>CGTATACG[4x]

In this study, we used d(CGTATACG)2, which forms a tetraplex base-pair junction that resembles the DNA–DNA contact structure, as a model target for two alkyl-linked diaminoacridine bis-intercalators, DA4 and DA5. To explore the possibility of targeting inter-DNA duplex structures, we synthesized two acridine-based derivatives, DA4 and DA5, by coupling 9-aminoacridine moieties with hydrocarbon chains of four and five atoms, respectively. Cross-linking of the junction site by the bis-intercalators induced substantial structural changes in the DNA, transforming it from a B-form helical end-to-end junction to an over-wounded side-by-side inter-duplex conformation with A-DNA characteristics and curvature. Furthermore, we have shown that the different topological changes induced by DA4 and DA5 lead to the inhibition of topoisomerase 2 activities, which may account for their antitumor effects.

To understand the structural basis of the binding of DA4 and DA5, we determined the crystal structures of DA4 and DA5 with the d(CGTATACG)2 sequence in the C2221 and P21 space groups, respectively, at a resolution of 1.58 Å. In contrast, the asymmetric unit of the DA5–DNA complex contains two independent duplexes, each intercalated by a single DA5 moiety and two Mg2+ ions, which form octahedral coordination with five water molecules and one phosphate oxygen from the thymine bases. In contrast to the unliganded DNA structure, the crystal assembly of the DA4–DNA and DA5–DNA complexes revealed that the duplexes were juxtaposed near terminal CpG sites (C1pG2 and C7*pG8*, respectively), with DA4 and DA5 bis-intercalating into neighboring duplexes. The four-carbon linker of DA4 adopted a relatively straight conformation, in contrast to the five-carbon linker of DA5, which bent toward the DNA backbone. In the DA4–DNA complex, the two chromophores formed an angle of ∼60° with the horizontal plane of the acridine ring, whereas in the DA5–DNA complex, the angle between the two acridine chromophores was ∼50°. This flexibility in the DA5 linker resulted in its chromophore aligning in an optimal position to form continuous stacking interactions with DNA base pairs. A detailed analysis revealed that, compared to DA4, the bending of the DA5 linker resulted in more π–π stacking interactions with DNA bases. Furthermore, amino nitrogen at carbon 9 of acridine in DA5 showed a direct water-mediated interaction with cytosines C1 and C9* from two adjacent duplexes. The bent linker and less tilted chromophore of DA5 bring the amino atoms closer to cytosines, favoring a direct water-mediated interaction which likely results in a more stable complex with stronger binding interactions. Our structural analysis of these complexes revealed that DA5, with its more flexible linker and increased DNA interactions exhibits a stronger TOP2 inhibitory and anticancer activities than DA4.> QTLPDISTFSQQQIFENWVQNRCIGKIADSKSLKEDADASAAAWLEASNLPAENFEKADEVIVSLLKQKVGGTEPGHYQILKCTLIANSDAIRPLKSSKHH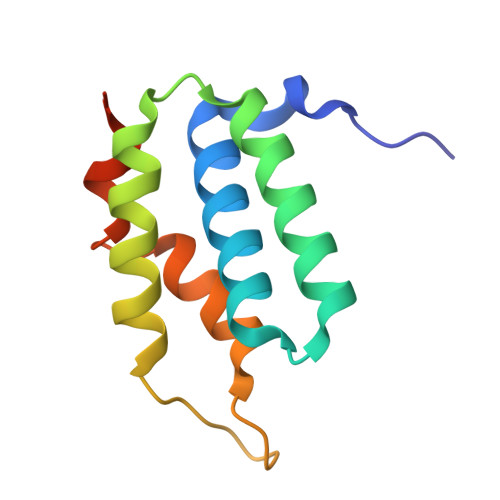HHHH>[2x]GSSKVCRGVIKLSSDCLNKMKLSDFVVLIREKYSYPQDISLLDASNQRLLFDYDFEDLNDRTLSEINLGNGSIILFSDEEGDTMIR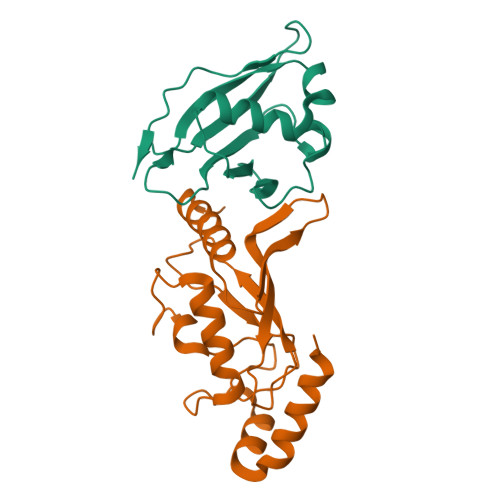KAIELFLDVDDELPCNTCSLPDVEVPLIKANNSPSKNEEEE;>[2x]GSMSSLCLQRLQEERKKWRKDHPFGFYAKPVKKADGSMDLQKWEAGIPGKEGTNWAGGVYPITVEYPNEYPSKPPKVKFPAGFYHPNVYPSGTICLSILNEDQDWRPAITLKQIVLGVQDLLDSPNPNSPAQEPAWRSFSRNKAEYDKKVLLQAKQYSK> EDHQRQVEAMLDDIRQLRKELLLNIAIIDEYIPVEHVELIEKYVSWSEEHGDWQLKAIAYTGNNMRASAPPAKKEFSNNNQTVPMYYSYRADLGASTAEHRPRTSSKKHRASIRL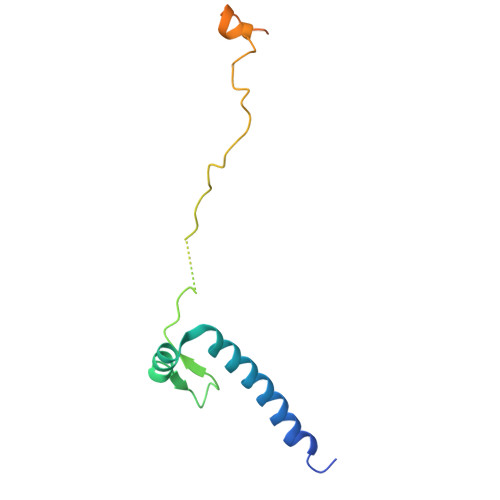QQLLT> MKAYMFPGQGSQAKGMGRALFDAFPALTARADGVLG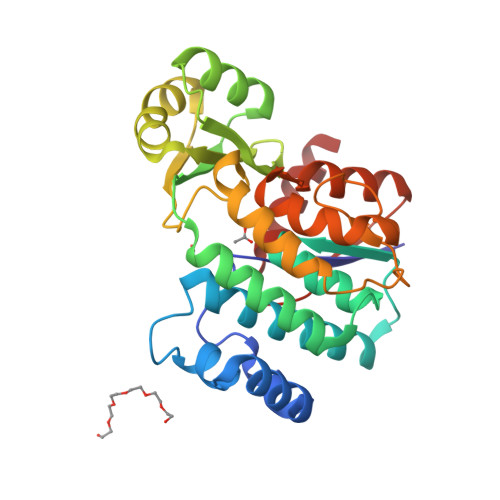YSIRALCQDDPDQRLSQTQFTQPALYVVNALSYLKRREEEAPPDFLAGHSLGEFSALFAAGVFDFETGLALVKKRGELMGDARGGGMAAVIGLDEERVRELLDQNGATAVDIANLNSPSQVVISGAKDEIARLQVPFEAAGAKKYTVLRVSAAFHSRFMRPAMVEFGRFLEGYDFAPPKIPVISNVTARPCKADGIRAALSEQIASPVRWCESIRYLMGRGVEEFVECGHGIVLTGLYAQIRRDA>[6x]SAMNNEGKALMAIKGSFSNLVNMLLDWDDVHNSDLCSWRGVFCDNVSYSVVSLNLSSLNLGGEISPAIGDLRNLQSIDLQGNKLAGQIPDEIGNCASLVYLDLSENLLYGDIPFSISKLKQLETLNLKNNQLTGPVPATLTQIPNLKRLDLAGNHLTGEISRLLYWNEVLQYLGLRGNMLTGTLSSDMCQLTGLWYFDVRGNNLTGTIPESIGNCTSFQILDISYNQITGEIPYNIGFLQVATLSLQGNRLTGRIPEVIGLMQALAVLDLSDNELVGPIPPILGNLSFTGKLYLHGNMLTGPIPSELGNMSRLSYLQLNDNKLVGTIPP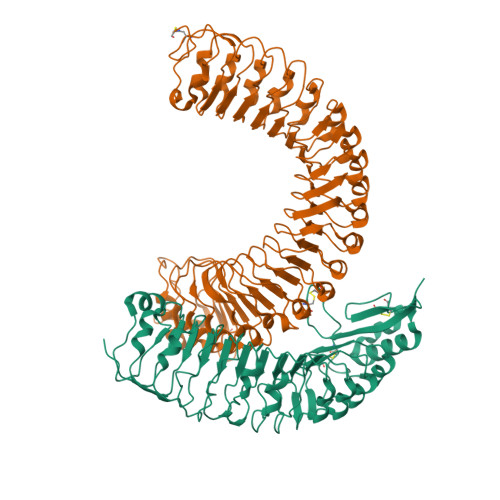ELGKLEQLFELNLANNRLVGPIPSNISSCAALNQFNVHGNLLSGSIPLAFRNLGSLTYLNLSSNNFKGKIPVELGHIINLDKLDLSGNNFSGSIPLTLGDLEHLLILNLSRNHLSGQLPAEFGNLRSIQMIDVSFNLLSGVIPTELGQLQNLNSLILNNNKLHGKIPDQLTNCFTLVNLNVSFNNLSGIVPPMKNFSRFAPASFVGNPYLCGNWVGSICGPHHHHHH;>[6x]TSDSTAPSALIDGPQTGFTMTNDGARTEPDEQDAVYDIMRATGNDWAAAIPDVCRGRWHGIECMPDQDNVYHVVSLSFGALSDDTAFPTCDPQRSYVSESLTRLKHLKALFFYRCLGRAPQRIPAFLGRLGSSLQTLVLRENGFLGPIPDELGNLTNLKVLDLHKNHLNGSIPLSFNRFSGLRSLDLSGNRLTGSIPGFVLPALSVLDLNQNLLTGPVPPTLTSCGSLIKIDLSRNRVTGPIPESINRLNQLVLLDLSYNRLSGPFPSSLQGLNSLQALMLKGNTKFSTTIPENAFKGLKNLMILVLSNTNIQGSIPKSLTRLNSLRVLHLEGNNLTGEIPLEFRDVKHLSELRLNDNSLTGPVPFERDTVWRMRRKLRLYNNAGLCVNRDSDLDDAFGSKSGSTVRLCDAETSRPAPSGTVQHLSREEDGAL>[2x]QPAHKASQSMITPTTQIAGAGVLGNDRKPDESCARAAAAADPGPPTRPAHNAAGVSPEMVQVPAEAQRIVVLSGDQLDALCALGLQSRIVAAALPNSSSSQPSYLGTTVHDLPGVGTRSAPDLR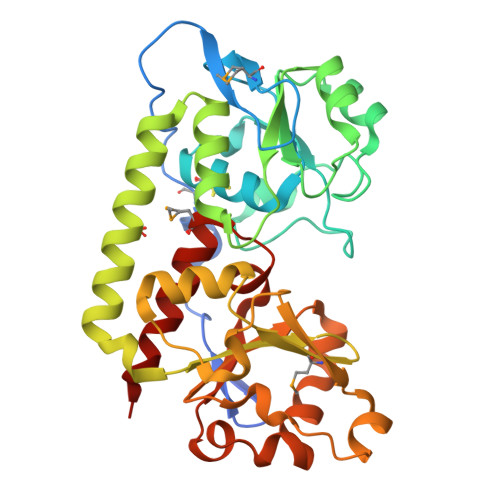AIAAAHPDLILGSQGLTPQLYPQLAAIAPTVFTAAPGADWENNLRGVGAATARIAAVDALITGFAEHATQVGTKHDATHFQASIVQLTANTMRVYGANNFPASVLSAVGVDRPPSQRFTDKAYIEIGTTAADLAKSPDFSAADADIVYLSCASEAAAERAAVILDSDPWRKLSANRDNRVFVVNDQVWQTGEGMVAARGIVDDLRWVDAPIN>GCCAGGAUGUUGGCUUAGAAGCAGCCAUCAUUU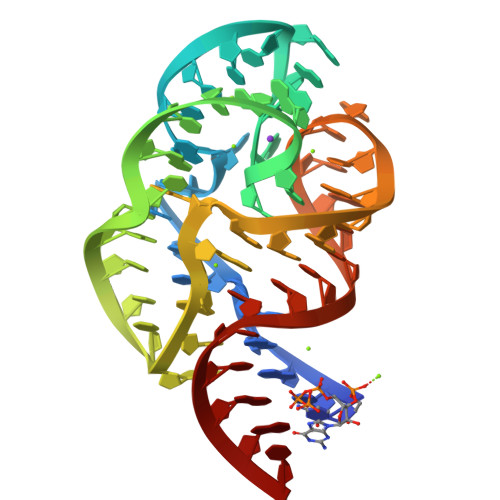AAAGAAAGCGUAAUAGCUCACUGGU[4x]AChBPs are homopentameric, water-soluble homologs of the ligand-binding domain of LGICs and well-established structural surrogates for nicotinic acetylcholine receptors (nAChR). Importantly, AChBPs can bind nAChR-specific ligands and induce similar conformational changes as in the membrane bound receptors. LGICs are activated by ligands binding at subunit interfaces of their extracellular domains, thereby inducing conformational changes that affect the structure of a central pore and its ability to transport ions through the membrane. Additional density was found in all structures at the interface between the subunits in the orthosteric agonist and antagonist binding site, next to loop C in which the respective ligands could be modelled.

In total, five structures of Ls-AChBP in complex with a ligand were successfully solved. The unit cell was comprised of two or four pentamers of Ls-AChBP in the presence of FL1613, FL1856, FL1888, FL3044, VUF24234 and VUF6105. However, the number of binding sites in which additional electron density was observed varied. The electron density in the binding site region was generally poor, indicating that compounds may have had several binding modes in the site. A computational alignment and superimposition of AChBP taken from the protein–ligand complexes and the apo structure showed that there were no large global conformational changes in any of the structures upon ligand binding. However, there were small changes in the loop C region of the crystal structures of Ls-AChBP. When comparing the protomers in complex with a ligand we observed that loop C moves differently upon binding of different compounds. Notably, binding of FL1888, VUF24234 and VUF6105 results in a movement of the loop closer to the compound, while binding of FL1856, FL3044, FL1613 and FL1909 does not have the same effect. The plot indicates that binding of nicotine, FL1613, FL1909, FL1856 and FL3044 do not result in any significant conformational changes in this region, while binding of FL1888, VUF24234 and VUF6105 do.

>[10x]MRRNIFCLACLWIVQACLSLDRADILYNIRQTSRPDVIPTQRDRPVAVSVSLKFINILEVNEITNEVDVVFWQQTTWSDRTLAWNSSHSPDQVSVPISSLWVPDLAAYNAISKPEVLTPQLARVVSDGEVLYMPSIRQRFSCDVSGVDTESGATCRIKIGSWTHHSREISVDPTTENSDDSEYFSQYSRFEILDVTQKKNSVTYSCCPEAYEDVEVSLNFRKKGRSEILGSHHHHHH> MSNWVMQEENKQGNLTPLFEELLQQCPPGGQNKTAHMVSAYQLAQGNWMPTSCHVFMGTISARRTKTHPYEAYVKLRELVEEHKMKTLCPGSSLGKHNDWIIGKIKYQGNLRTKHMLNPGKVAEQLCREGHRHNVYNKTIGSVMTATGIRLEKLPVVRAQTDTTNFHQAIRDKIDKEENLQTPGLHKKLMEVFNALKRPELESSYDAVEWEELERGINRKGAAGFFERKNIGEILDSEKNKVEEIIDNLKKGRNIKYYETAIPKNEKRDVNDDWTAGDFVDEKKPRVIQYPEAKTRLAITKVMYKWVKQKPVVIPGYEGKTPLFQIFDKVKKEWDQFQNPVAVSFDTKAWDTQVTTKDLELIKDIQKYYFKKKWHKFIDTLTMHMTEVPVICADGEVYIRKGQRGSGQPDTSAGNSMLNVLTMVYAFCEATGVPYKSFDRVAKIHVCGDDGFLITERALGEKFASKGVQILYEAGKPQKITEGDKMKVAYQFDDIEFCSHTPIQVRWSDNTSSYMPGRNTTTILAKMATRLDSSGERGTIAYEKAVAFSFLLMYSWNPLIRRICLLVLSTELQVKPGKSTTYYYEGDPISAYKEVIGHNLFDLKRTSFEKLAKLNLSMSVLGAWTRHT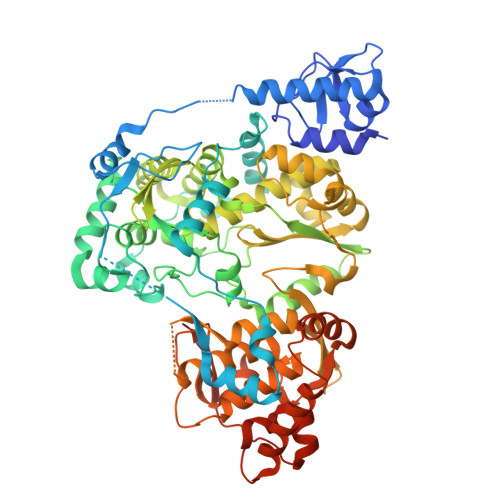SKRLLQDCVNMGVKEGNWLVNADRLVSSKTGNRYIPGEGHTLQGRHYEELVLARKGSSSHHHHHH> MEDINFASLAPRHGSRPFMGTWNEIGTSQLNGGAFSWSS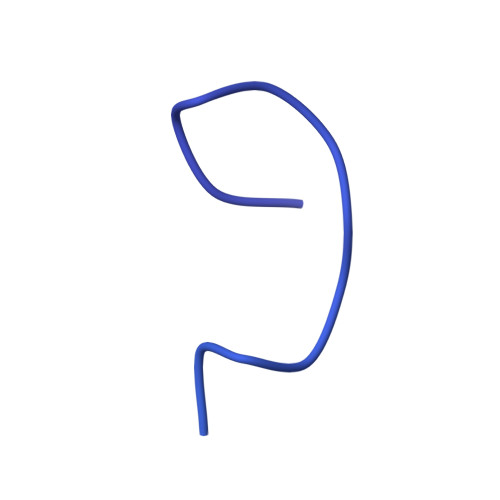LWSGIKNFGSSIKSFGNKAWNSNTGQMLRDKLKDQNFQQKVVDGLASGINGVVDIANQALQNQINQRLENSRQPPVALKQRPTPEPEEVEVEEKLPPLETAPPLPSKGEKRPRPELEETLVVESREPPSYEQALKEGASYPMTRPIGSMARPVYGKEKTPVTLELPPPAPTVPPMPTPTLGTNVPRLAAPTVAVATPARRVRGANWQSTLNSIVGLGVKSLKRRRCY>SSPGKPPRLVGGPMDASVEEEGVRRALDFAVGEYNKASNDMYHSRALQVVRARKQINAGVNYFLDVELGRTTCT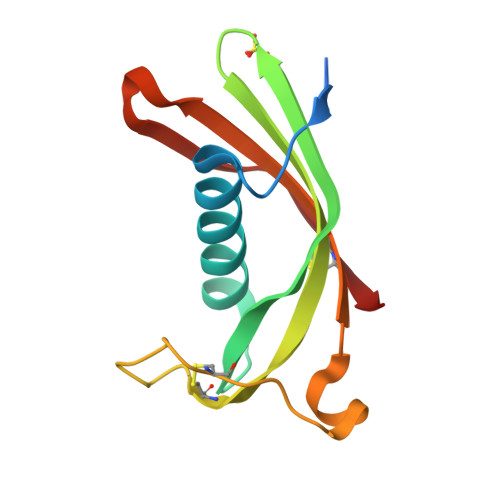KTQPNLDNCPFHDQPHLKRKAFCSFQIYAVPWQGTMTLSKSTCQDA[2x]>LIQERRSHEVNPAAHLTGANSSLTGSGGPLLWETQLGLAFLRGLSYHDGALVVTKAGYYYIYSKVQL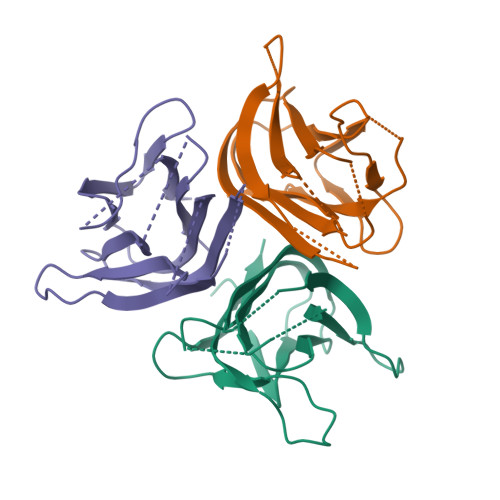GGVGCPLGLASTITHGLYKRTPRYPEELELLVSQQSPCGRATSSSSNWFDSSFLGGVVHLEAGEEVVVRVLDERLVRLRDGTRSYFGAFMV[3x]> MQSQPQQLQQQQLQQQQLLQQSQLLQPQYFEKQQIADYIDKTFEKKIKEWKTWTFSSVFIIFLPLLLFQMLFLSFMFSPSPKSTSTSMISVILRTTGNHIFGIILYVIGQLILGASYHSICSVYRQVPASFKEQFTVLSIPHLIFITLNTLIQPLFLYFFFSIPLNKFSLSSIIEVCYQDFSETIPVAKCELEYNLFFYLFVLSCIGLVCSGLFRIYSNQEFVYSFPKANIPTFIQIKSMLYNNFWISFYTSFYLFFLGSFLLGILFLILFKTFTIQILIFSIKLWCFTFAIIFQNLTRNRLFEIYFTRGLRFTLETFNSVTFDSSNSQQQQQQQQQPQQQQQQQQQTLFDNKPIIENGSIFLLKAIYSCDPLIQALGWKDFLHLSKYSQPRRTYLYREMSELLDQPSILKIIRQYEDQINDLSLKLSCPREYYESLNSGNIKKEDDKNKNSNNNNNNNNNNNNNNNNNNNNNNSNNNNNSIIFKIGNNIEKIIKKTLNFISGVKFDYNLYECEIRQALSNTQSILWSIESIGSLIVSAQIND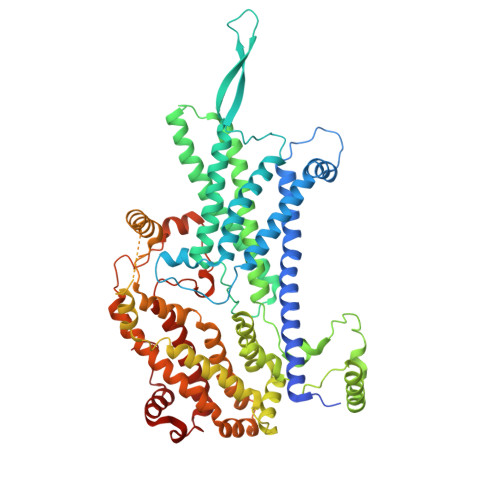DRETMELLHRYQIPQKFLIPLFQILALIDQLEKDLSHQIELDKFTINRDYYFLKSFSNLIEPPLNCLGILKTSRPHFRIFKLVGKNMISQVLETIGHQISDISFPYDLRTTLNSYRNGEFSIYQ>[2x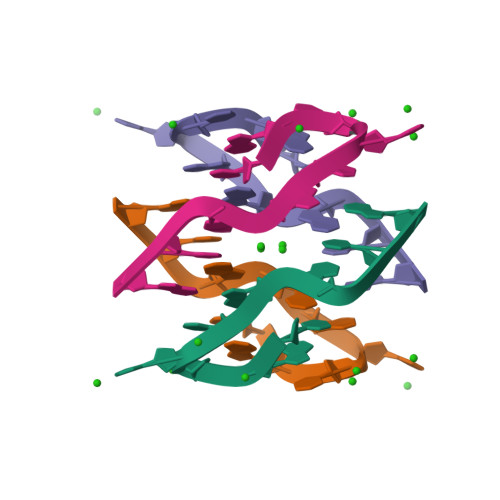]CGTTAGGCG> VFHKIRNEDLIFNESLGQGTFTKIFKGVRREVGDYGQLHETEVLLKVLDKAHRNYSESFFEAASMMSKLSHKHLVLNYGVCVCGDENILVQEFVKFGSLDTYLKKNKNCINILWKLEVAKQLAAAMHFLEENTLIHGNVCAKNILLIREEDRKTGNPPFIKLSDPGISITVLPKDILQERIPWVPPECIENPKNLNLATDKWSFGTTLWEICSGGDKPLSALDSQRKLQFYEDRHQLPAPKAAELANLINNCMDYEPDHRPSFRAIIRDLNSLFTPDLVPRGSHHHHHH

JAK2, like other JAK family members, comprises a catalytically active C-terminal tyrosine kinase domain (JH1), a regulatory pseudokinase domain (JH2), and a Src homology-2 (SH2)-like domain that, together with the N-terminal FERM (N-terminal 4.1, ezrin, radixin, moesin) domain, forms the major receptor interaction moiety. The JH2 domain has a key role in mediating both negative and positive regulation of JAK kinase activity and numerous disease mutations locate in JH2, including the prevalent hyperactivating JAK2 V617F in MPN. Previous studies have demonstrated that JAK2 JH2 binds ATP and possesses regulatory autophosphorylation activity on Ser523 and Tyr570. To gain insights on the compound binding modes to JAK2 JH2 and to analyze whether any differences could be observed between binding to WT and V617F, we determined the crystal structures of selected small molecules with JAK2 JH2 WT and V617F.

Our diaminotriazine hits share the aminoanilinyltriazine core structure and were confirmed to have JH2-selectivity over JH1. Diaminotriazine compounds 23–33 were found to bind JAK2 JH2 domain generally with selectivity over JH1, except for analog 33, which bound JH1 domain more effectively than JH2. In general, the binding of diaminotriazine analogs was stronger to JH2 domain of JAK1 compared to JH2 domain of JAK2. Data in the present study and that by Jorgensen group indicate that aminoanilinyltriazine compounds might possess slightly (2- to 3-fold) stronger binding to V617F than wild-type. All compounds anchor to the hinge region and extend towards the Gln626 gatekeeper and towards the G-loop. Overall, the binding modes are highly similar between WT and V617F structures and no major differences can be seen that would explain the differences in the observed IC50 values.>MTNLPMNKLIDEVNNELSVAINKSVMDTQLEESMLYSLNAGGKRIRPVLLLLTLDSLNTEYELGMKSAIALEMIHTYSLIHDDLPAMDNDDYRRGKLTNHKVYGEWTAILAGDALLTKAFELISSD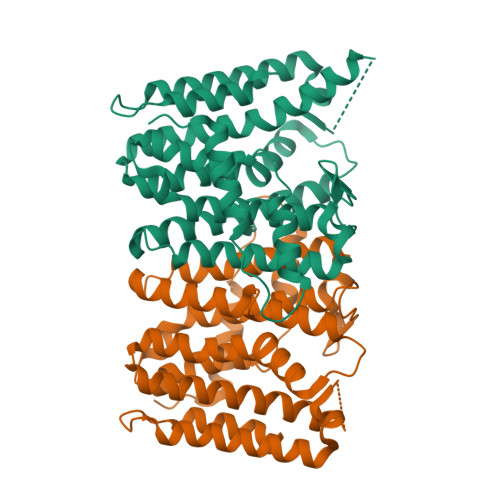DRLTDEVKIKVLQRLSIASGHVGMVGGQMLDMQSEGQPIDLETLEMIHKTKTGALLTFAVMSAADIANVDDTTKEHLESYSYHLGMMFQIKDDLLDCYGDEAKLGKKVGSDLENNKSTYVSLLGKDGAEDKLTYHRDAAVDELTQIDEQFNTKHLLEIVDLFYSRDHKGHHHHHH[2x]> MALTLVEQILAEFQLQEEDLKKVMRRMQKEMDRGLRLETHEEASVKMLPTYVRSTPEGSEVGDFLSLDLGGTNFRVMLVKVGEGEEGQWSVKTKHQMYSIPEDAMTGTAEMLFDYISECISDFLDKHQMKHKKLPLGFTFSFPVRHEDIDKGILLNWTKGFKASGAEGNNVVGLLRDAIKRRGDFEMDVVAMVNDTVATMISCYYEDHQCEVGMIVGTGCNACY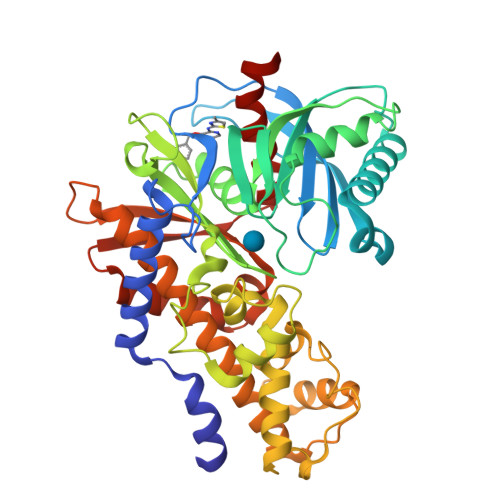MEEMQNVELVEGDEGRMCVNTEWGAFGDSGELDEFLLEYDRLVDESSANPGQQLYEKLIGGKYMGELVRLVLLRLVDENLLFHGEASEQLRTRGAFETRFVSQVESDTGDRKQIYNILSTLGLRPSTTDCDIVRRACESVSTRAAHMCSAGLAGVINRMRESRSEDVMRITVGVDGSVYKLHPSFKERFHASVRRLTPSCEITFIESEEGSGRGAALVSAVACKKACMLGQ>VTALSRLGEPPSGHDGNSEVRRIAMKRATVPVLRRVAAVCAAALLVTVGTGGPASATGTRSAICRATTVEVTLGKGTGKMWGELCRPAGSSPDTVVTMVHGATYNHNYWDFPYQPDKYSFRKMLNGAGYATFVVDRLGTGNSTVPPSSELNLTVEARQMHEVVQGLRTGRIGGTGFGKVVLAGYALGSAVTSIEASTFHDVDAVLITALGHYNNPAGTQAIIDNGLSPNDDPVLKDRHHYDDGYATTKPGSRKHVFYADRPMDPGVLATDELTKDANVFTEAADPLVIDPAVSRAIDVPVMFALGDRDPLMCGDGYEDCSSQAALRAQEAPFWTSAPSFDVILVEDAGHGLNLVPNTRVYQDASRDWLDRVVGHGLEHHHHHH[7x]

StnA is an essential enzyme in the Streptonigrin biosynthesis pathway. The crystal structure shows that StnA has an α-helical cap domain positioned atop a common α/β hydrolase domain. The data clearly shows that Ser185-Asp308-His349 constitutes the catalytic triad of StnA.

The S185A complex structure was determined in a different space group P1 with the resolution of 2.90 Å by molecular replacement, using SeMet-StnA as a search model, with 7 molecules in the asymmetric unit. The electron density for the substrate at the binding pocket is clear in every molecule of the asymmetric unit. Substrate 4 (PDB 3-letter-code is STM) perfectly binds into this narrow pocket. Among the four hydrogen bonds, two hydrogen bonds are between the substrate and the main chain amide nitrogen of Ala102 and Leu186 (2.7 Å and 3.1 Å respectively) and play key roles in forming the oxyanion hole. Two additional hydrogen bonds are between the main-chain carbonyl group of Ala282 and the hydroxyl group of ring D, and between the side-chain amide group of Asn277 and the carbonyl group of ring A. Furthermore, there is also a possible π-π stacking interaction between ring A and Phe279. The hydrophobic nature of the binding sites and the aromatic nature of the substrate suggest that the substrate recognition could be predominantly controlled by the shape-complementarity between the substrate and the binding pocket, i.e. hydrophobic interactions. The surface view shows that the binding interaction between STM and StnA is mainly contributed by the cap domain residues. The His349 Nδ1 atom forms a hydrogen bond/salt bridge with Oδ1 (3.2 Å) and Oδ2 (2.7 Å) of Asp308, located between strand β7 and helix αE. The alignment between native and S185A mutant complex was shown in Supplementary Fig. S3. The figure suggests that the catalytic triad is relative stable with small change.3-[3-(4-chlorophenyl)-1,2,4-oxadiazol-5-yl]propan-1-ol | C11 H11 Cl N2 O2 | 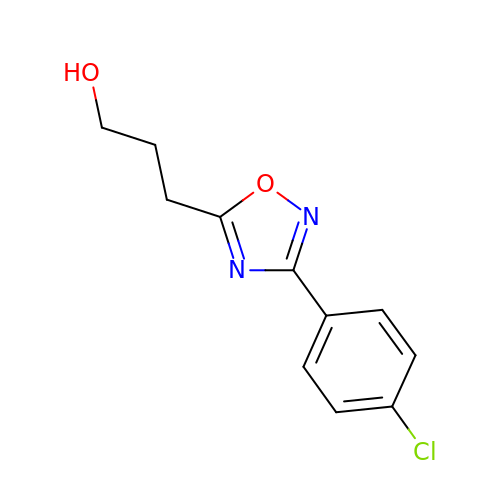BTURSBZSHDJVMU-UHFFFAOYSA-N>ATHEVHMLNKGESGAMVFEPAFVRAEPGDVINFVPTDKSHNVEAIKEILPEGVESFKSKINESYTLTVTEPGLYGVKCTPHFGMGMVGLVQVGDAPENLDAAKTAKMPAK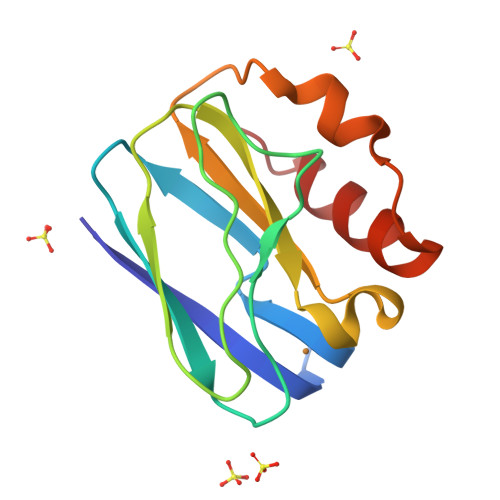ARERMDAELAQVN[2x]>MIDVSSQRVNVQ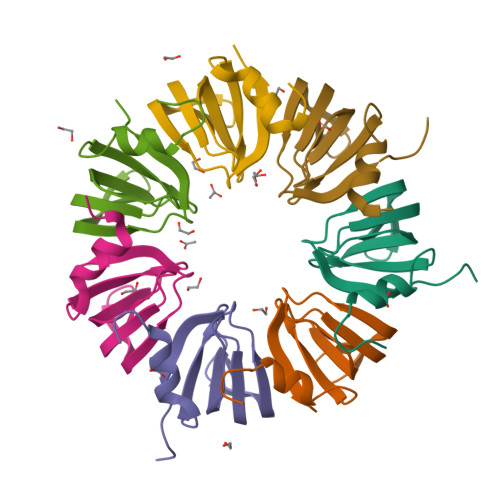RPLDALGNSLNSPVIIKLKGDREFRGVLKSFDLHMNLVLNDAEELEDGEVTRRLGTVLIRGDNIVYISRGKLAA[7x]> MLETRATTAKQLVQAPEQPAPQPEVAPPTTEQPAPAPAPGTTPGTENFNTPNATPETTEPRVLVSEVLVRPQSGQLTPELETQVYNVIRTQPGRTTTRSQLQEDINAIFGTGFFSNVQASPEDTPLGVRVSFIVQPNPVLSKVEIQANPGTNVPSVLPQATADEIFRAQYGKILNLRDLQEGIKELTKRYQDQGYVLANVVGAPQ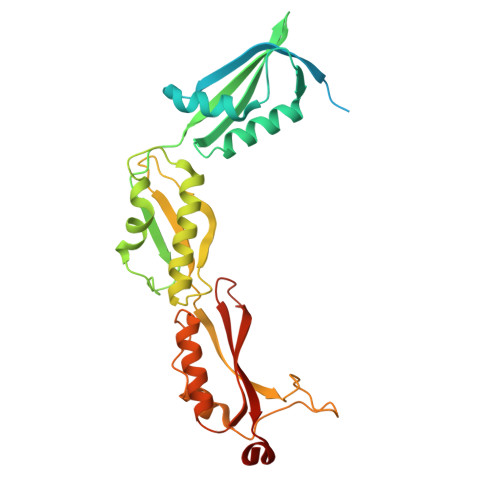VSENGVVTLQVAEGVVENISVRFRNKEGQDVNEQGQPIRGRTQDYIITREVELKPGQVFNRNTVQKDLQRVFGTGLFEDVNVSLDPGTDPTKVNVVVNVVERSLEHHHHHH>MTQSSQDTTVSPVVAASQNSWRCVQSGDREGWLALMADDIVVEDPIGEAVTNPDGTGV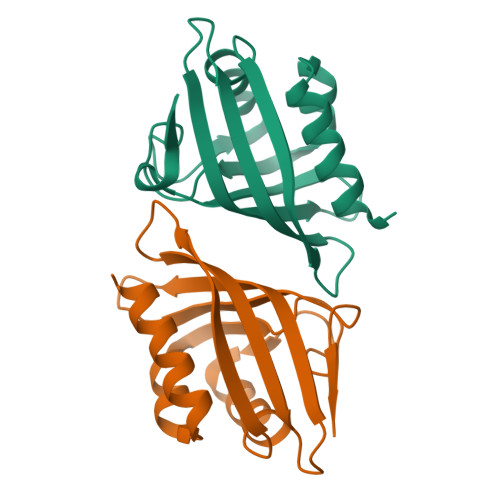RGKAALAAFYDTNIGPNRLRVTCEATFPSSSPTEIAYILVLETTFPNGFVATVRGVFTYRVDDAGLITNLRGYWNMDAMTFTEAPDR[8x]> IIGGRESRPHSR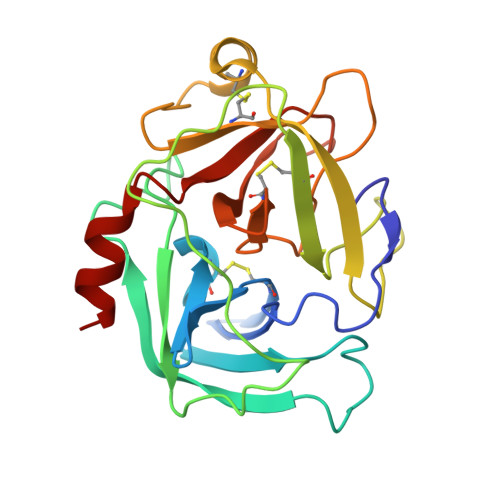PYMAYLQIQSPAGQSRCGGFLVREDFVLTAAHCWGSNINVTLGAHNIQRRENTQQHITARRAIRHPQYNQRTIQNDIMLLQLSRRVRRNRNVNPVALPRAQEGLRPGTLCTVAGWGRVSMRRGTDTLREVQLRVQRDRQCLRIFGSYDPRRQICVGDRRERKAAFKGDSGGPLLCNNVAHGIVSYGKSSGVPPEVFTRVSSFLPWIRTTMR(5S,6S)-5-[(1-carboxyethenyl)oxy]-6-hydroxycyclohexa-1,3-diene-1-carboxylic acid | C10 H10 O6 | 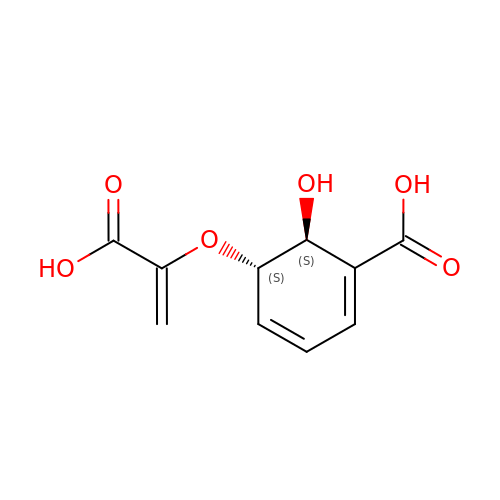NTGWPRCCOQCMGE-YUMQZZPRSA-N>[2x]SPILGYWKIKGLVQPTRLLLEYLEEKYEEHLYERDEGDKWRNKKFELGLEFPNLPYYIDGDVKLTQSMAIIRYIADKHNMLGGCPKERAEISMLEGAVLDIRYGVSRIAYSKDFETLKVDFLSKLPEMLKMFEDRLCHKTYLNGDHVTHPDFMLYDALDVVLYMDPMCLDAFPKLVCFKKRIEAIPQIDKYLKSSKYIAWPLQGWQATFGGGDHPPKSDEFVIEKSLNRIKKFWKEAQYEVIEHSSGLKLVREWDVLEQACKEDLEELVSMKASNYYKIFEQDCLDLESKLTKLSEIQVNWVEVQFYWLDLYGILGENLDIQNFLPLETSKFKSLTSEYKMITTRAFQLDTTIEVIHIPNFDTTLKLTIDSLKMIKSSLSTFLERQRRQFPRFYFLGNDDLLKIIGSGKHHDQVSKFMKKMFGSIESIIFLEDFITGVRSVEGEVLNLNEKIELKDSIQAQEWLNILDTEIKLSVFTQFRDCLG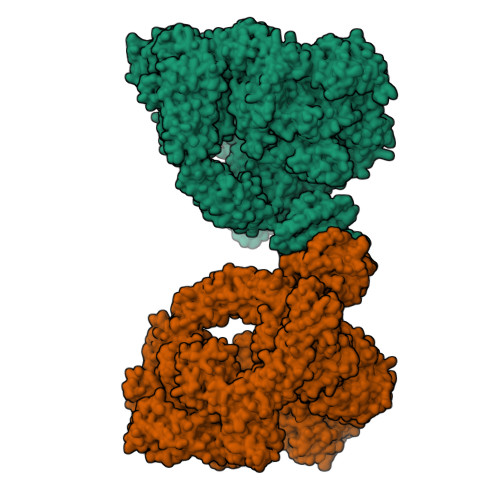QIKDGTDIEVVVSKYIFQAILLSAQVMWTELVEKCLQTNQFSKYWKEVDMKIKGLLDKLNKSSDNVKKKIEALLVEYLHFNNVIGQLKNCSTKEEARLLWAKVQKFYQKNDTLDDLNSVFISQSGYLLQYKFEYIGIPERLIYTPLLLIGFATLTDSLHQKYGGCFFGPAGTGKTETVKAFGQNLGRVVVVFNCDDSFDYQVLSRLLVGITQIGAWGCFDEFNRLDEKVLSAVSANIQQIQNGLQVGKSHITLLEEETPLSPHTAVFITLNPGYNGRSELPENLKKSFREFSMKSPQSGTIAEMILQIMGFEDSKSLASKIVHFLELLSSKCSSMNHYHFGLRTLKGVLRNCSPLISEFGEGEKTVVESLKRVILPSLGDTDELVFKDELSKIFDSAGTPLNSKAIVQCLKDAGQRSGFSMSEEFLKKCMQFYYMQKTQQALILVGKAGCGKTATWKTVIDAMAIFDGHANVVYVIDTKVLTKESLYGSMLKATLEWRDGLFTSILRRVNDDITGTFKNSRIWVVFDSDLDPEYVEAMNSVLDDNKILTLPNGERLPIPPNFRILFETDNLDHTTPATITRCGLLWFSTDVCSISSKIDHLLNKSYEALDNKLSMFELDKLKDLISDSFDMASLTNIFTCSNDLVHILGVRTFNKLETAVQLAVHLISSYRQWFQNLDDKSLKDVITLLIKRSLLYALAGDSTGESQRAFIQTINTYFGHDSQELSDYSTIVIANDKLSFSSFCSEIPSVSLEAHEVMRPDIVIPTIDTIKHEKIFYDLLNSKRGIILCGPPGSGKTMIMNNALRNSSLYDVVGINFSKDTTTEHILSALHRHTNYVTTSKGLTLLPKSDIKNLVLFCDEINLPKLDKYGSQNVVLFLRQLMEKQGFWKTPENKWVTIERIHIVGACNPPTDPGRIPMSERFTRHAAILYLGYPSGKSLSQIYEIYYKAIFKLVPEFRSYTEPFARASVHLYNECKARYSTGLQSHYLFSPRELTRLVRGVYTAINTGPRQTLRSLIRLWAYEAWRIFADRLVGVKEKNSFEQLLYETVDKYLPNQDLGNISSTSLLFSGLLSLDFKEVNKTDLVNFIEERFKTFCDEELEVPMVIHESMVDHILRIDRALKQVQGHMMLIGASRTGKTILTRFVAWLNGLKIVQPKIHRHSNLSDFDMILKKAISDCSLKESRTCLIIDESNILETAFLERMNTLLANADIPDLFQGEEYDKLLNNLRNKTRSLGLLLDTEQELYDWFVGEIAKNLHVVFTICDPTNNKSSAMISSPALFNRCIINWMGDWDTKTMSQVANNMVDVIPMEFTDFIVPEVNKELVFTEPIQTIRDAVVNILIHFDRNFYQKMKVGVNPRSPGYFIDGLRALVKLVTAKYQDLQENQRFVNVGLEKLNESVLKVNELNKTLSISLVKSLTFEKERWLNTTKQFSKTSQELIGNCIISSIYETYFGHLNERERADMLVILKRLLGKFAVKYDVNYRFIDYLVTLDEKMKWLECGLDKNDYFLENMSIVMNSQDAVPFLLDPSSHMITVISNYYGNKTVLLSFLEEGFVKRLENAIRFGSVVIIQDGEFFDPIISRLISREFNHAGNRVTVEIGDHEVDVSGDFKLFIHSCDPSGDIPIFLRSRVRLVHFVTNKESIETRIFDITLTEENAEMQRKREDLIKLNTEYKLKLKNLEKRLLEELNNSQGNMLENDELMVTLNNLKKEAMNIEKKLSESEEFFPQFDNLVEEYSIIGKHSVKIFSMLEKFGQFHWFYGISIGQFLSCFKRVFIKKSRETRAARTRVDEILWLLYQEVYCQFSTALDKKFKMIMAMTMFCLYKFDIESEQYKEAVLTMIGVLSESSDGVPKLTVDTNNDLRYLWDYVTTKSYISALNWFKNEFFVDEWNIADVVANSDNNYFTMASERDVDGTFKLIELAKASKESLKIIPLGSIENLNYAQEEISKSKIEGGWILLQNIQMSLSWVKTYLHKHVEETKAAEEHEKFKMFMTCHLTGDKLPAPLLQRTDRFVYEDIPGILDTVKDLWGSQFFTGKISGVWSVYCTFLLSWFHALITARTRLVPHGFSKKYYFNDCDFQFASVYLENVLATNSTNNIPWAQVRDHIATIVYGGKIDEEKDLEVVAKLCAHVFCGSDNLQIVPGVRIPQPLLQQSEEEERARLTAILSNTIEPADSLSSWLQLPRESILNYERLQAKEVASSTEQLLQEM(3E,5E)-6-(3-{2-[3,4-bis(hydroxymethyl)phenyl]ethyl}phenyl)-1,1,1-trifluoro-2-(trifluoromethyl)octa-3,5-dien-2-ol 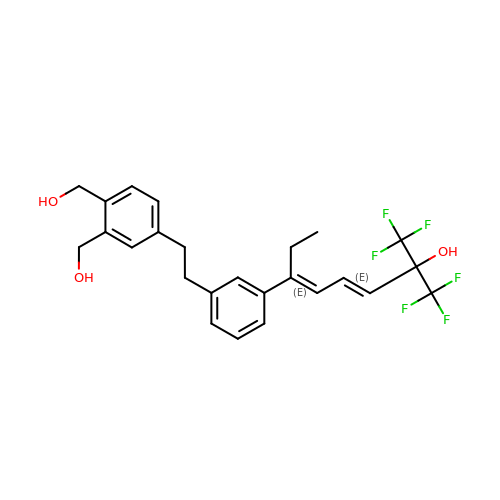| C25 H26 F6 O3 | GDMSFPQHUTVPQR-XFNPMVETSA-N>MATAEVLNIGKKLYEGKTKEVYELLDSPGKVLLQSKDQITAGNAARKNHLEGKAAISNKITSCIFQLLQEAGIKTAFTRKCGETAFIAPQCEMIPIEWVCRRIATGSFLKRNPGVKEGYKFYPPKVELFFKDDANNDPQWSEEQLIAAKFCFAGLLIGQTEVDIMSHATQAIFEILEKSWLPQNCTLVDMKIEFGVDVTTKEIVLADVIDNDSWRLWPSGDRSQQKDKQSYRDLKEVTPEGLQMVKKNFEWVAERVELLLKSESQCRVVVLMGSTSDLGHCEKIKKACGNFGIPCELRVTSAHKGPDETLRIKAEYEGDGIPTVFVAVAGRSNGLGPVMSGNTAYPVISCPPLT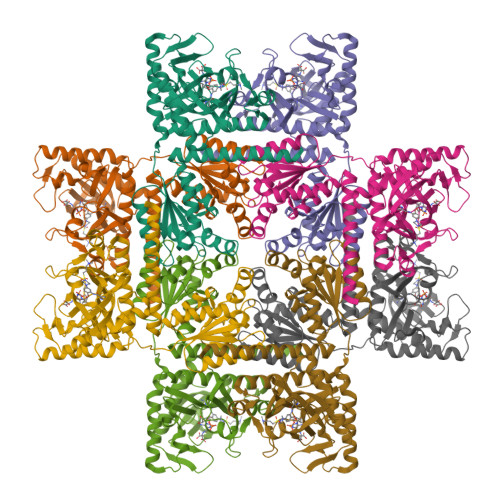PDWGVQDVWSSLRLPSGLGCSTVLSPEGSAQFAAQIFGLSNHLVWSKLRASILNTWISLKQADKKIRECNL[2x]(2R)-4-[1-(2-amino-5-chloropyrimidin-4-yl)-2,3-dihydro-1H-indol-6-yl]-2-(1,3-thiazol-2-yl)but-3-yn-2-ol 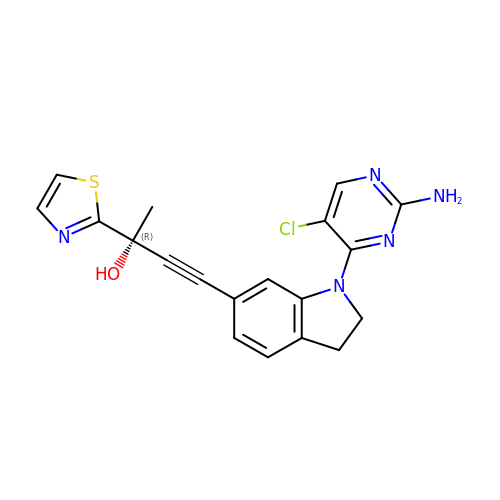| C19 H16 Cl N5 O S | OKFYOOFXVBCIIP-LJQANCHMSA-N> SQPDPAEEQKRVAAE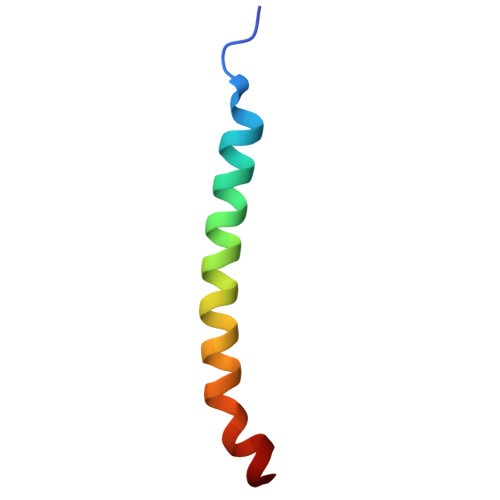VRFNFILFGAVIAAVRLAPIVLKH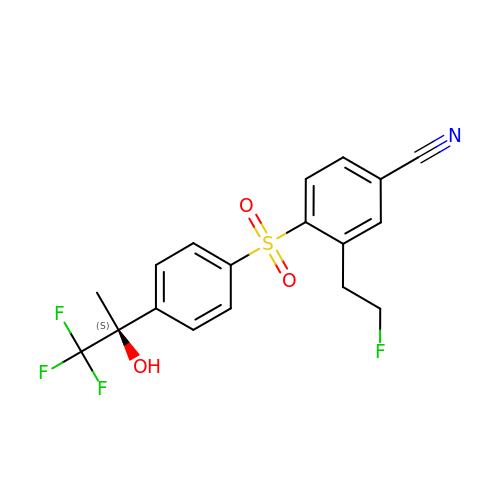3-(2-fluoroethyl)-4-({4-[(2S)-1,1,1-trifluoro-2-hydroxypropan-2-yl]phenyl}sulfonyl)benzonitrile | C18 H15 F4 N O3 S | HRHAWLGWRWLWQL-KRWDZBQOSA-N>ASHMFRKLAAESFGTFWLVFGGSGSAVLAAGFPELGIGFAGVALAFGLTVLTMAFAVGHISGGHFNPAVTIGLWAGGRFPAKEVVGYVIAQVVGGIVAAALLYLIASGKTGFDAAASGFASNGYGEHSPGGYSMLSALVVELVLSAGFLLVI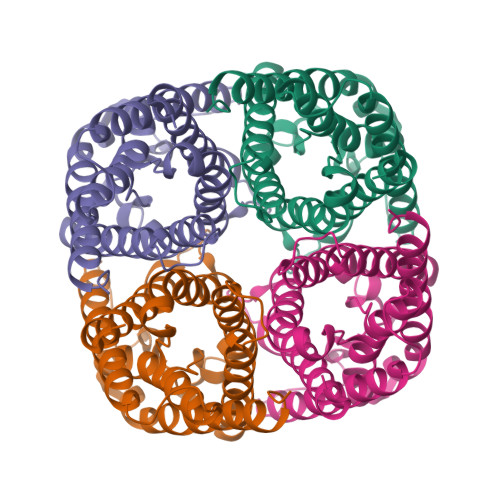HGATDKFAPAGFAPIAIGLACTLIHLISIPVTNTSVNPARSTAVAIFQGGWALEQLWFFWVVPIVGGIIGGLIYRTLLEKRD[2x]> SGTTNTVAAYNLTWKSTNFKTILEWEPKPVNQVYTVQ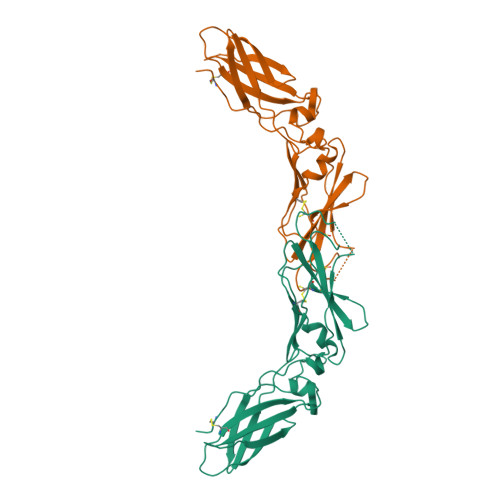ISTKSGDWKSKCFYTTDTECDLTDEIVKDVKQTYLARVFSYPAGNVESTGSAGEPLYENSPEFTPYLETNLGQPTIQSFEQVGTKVNVTVEDERTLVRRNNTFLSLRDVFGKDLIYTLYYWKSSSQEKGEFRSGKKTAKTNTNEFLIDVDKGENYCFSVQAVIPSRTVNRKSTDSPVECMG4-ACETYL-L-PHENYLALANINE 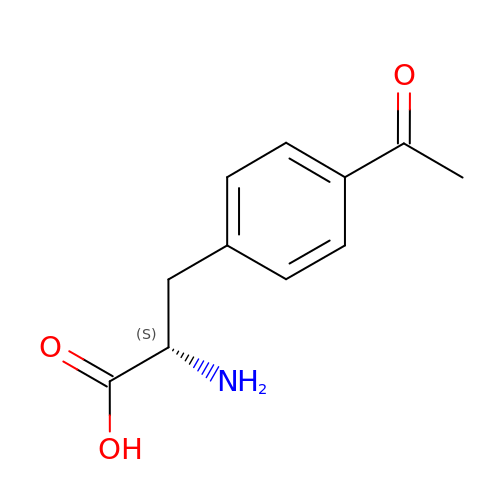| C11 H13 N O3 | ZXSBHXZKWRIEIA-JTQLQIEISA-N> GPHMQ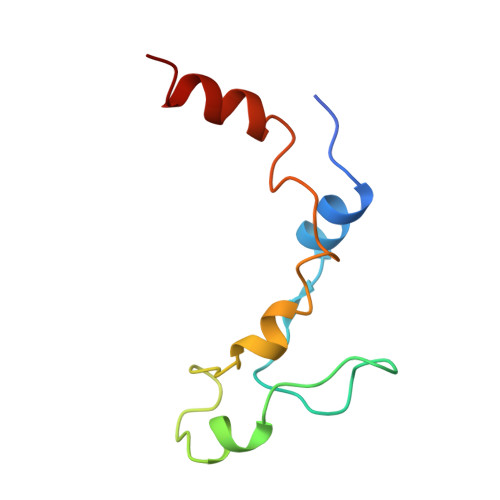PSAALQSLRSARFLPGIVQDIYPPGIKSPNPALNEAVQKKGRIFKYDVQFLLQFQNVFTEKPSPDFDQQVKALIGD>[2x]GSPEEIGL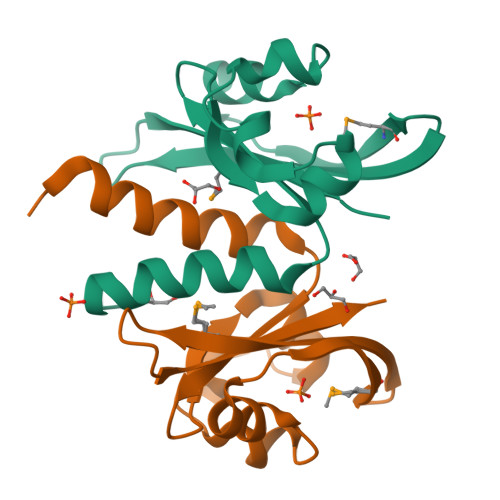LYQEKQAILEAIREGIVAINQEGTITMVNQTALKLLGYDNERNVLGTPILQLIPHSRLPEVIRTGQAEYDDEMVLGGETVIANRIPIKNKQGRVIGAVSTFRNK> ETGCNKALCASDVSKCLIQELCQCRPGEGNCSCCKECMLCLGALWDECCDCVGMCNPRNYSDTPPTSKSTVEELHEPIPSLFRALTEGDTQLNWNIVSFPVAEELSHHENLVSFLETVNQPHHQNVSVPS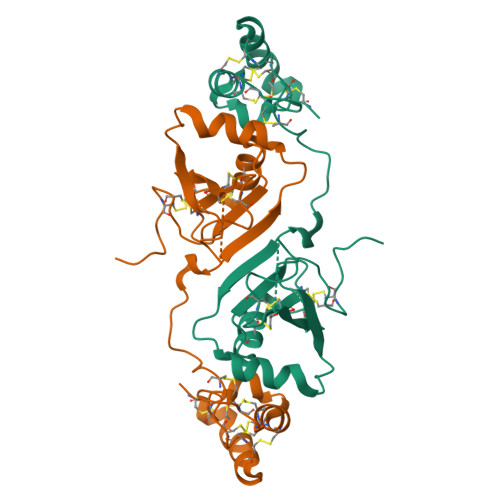NNVHAPYSSDKEHMCTVVYFDDCMSIHQCKISCESMGASKYRWFHNACCECIGPECIDYGSKTVKCMNCMFGTKHHHHHH> MIGMDRRSGLPLSGLAHLKQSVEDILTTPLGSRRMRPEYGSKLRRMVDMPVSEGWKSAVQAEVARSLGRWEPRIGLSAVRVVAVVDGRVDLLLSGVFEGENIN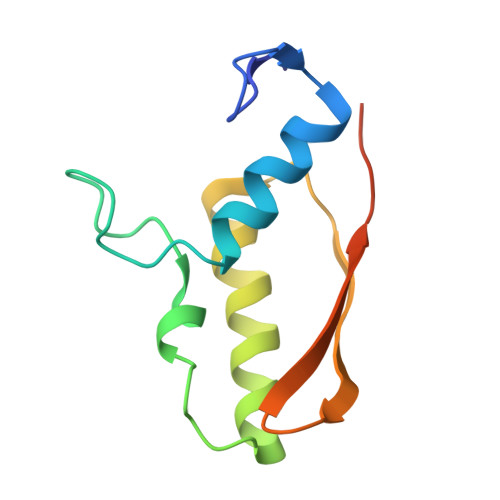MEVSA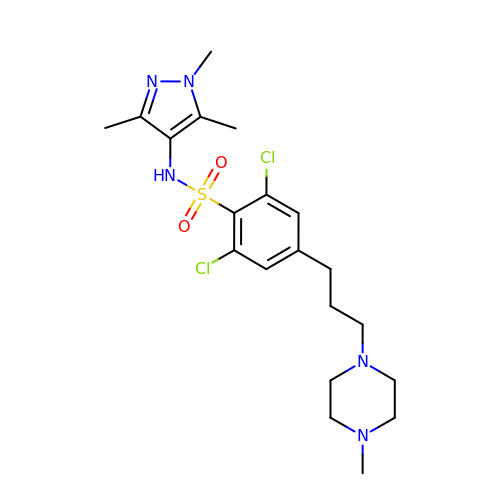2,6-dichloro-4-[3-(4-methylpiperazin-1-yl)propyl]-N-(1,3,5-trimethyl-1H-pyrazol-4-yl)benzenesulfonamide | C20 H29 Cl2 N5 O2 S | REQUPDWBGITKAD-UHFFFAOYSA-N>[3x]SKVVYVSH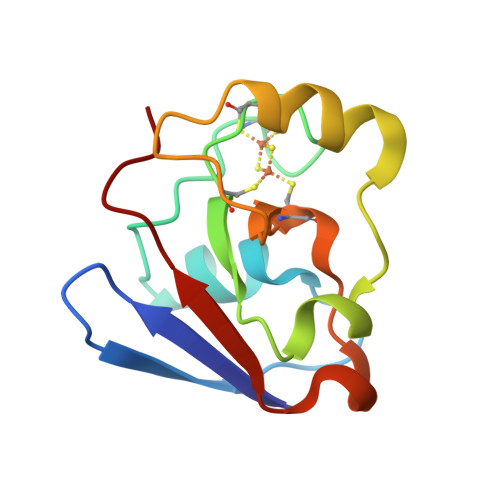DGTRRELDVADGVSLMQAAVSNGIYDIVGDCGGSASCATCHVYVNEAFTDKVPAANEREIGMLESVTAELKPNSRLCCQIIMTPELDGIVVDVPDRQW>MAHHHHHHMSSTLNTRLIWIDLEMTGLDTDNDQIIEIATIITDDHLNVLAEGPVLAIHQPDRILNAMDEWNTRQHGQSGLIERVRRSKLTARDAELQTLEFLKKWVNPKVSPMCGNSICQDRRFLHRLMPELEQYFHYRNLDVSTVKEL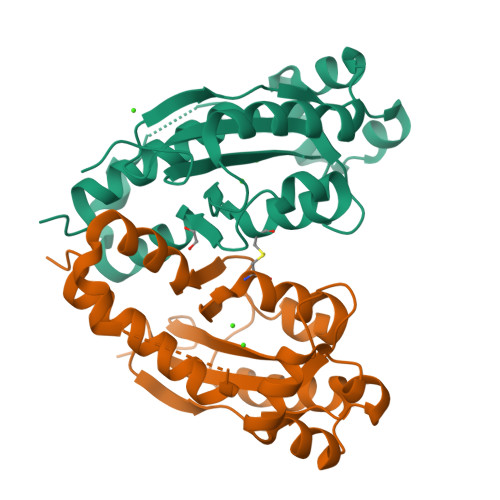SKRWRPEIMSGLKKNASHLAMDDIRDSISELKYYREYFFIMNTDGKD[6x]> DAILDEIDDVLEENAEEFVRSYIQ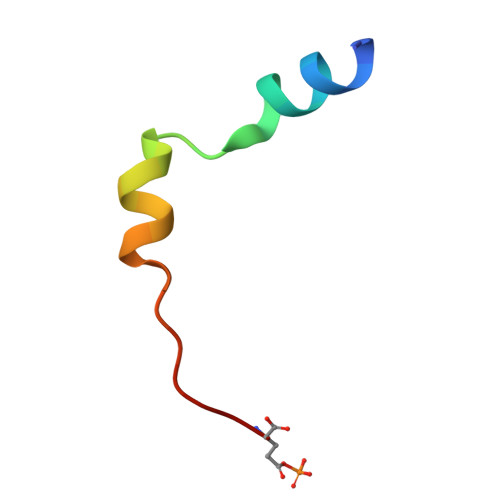KGGE> GIYQHFSIEDRPFLDKGMEWIKKVEDSYAPFLTPFINPHQEKLLKILAKTYGLACSSSGEFVSSEYVRVLLYPDYFQPEFSDFEISLQEIVYSNKFEYLTHAKILGTVINQLGIERKLFGDILVDEERAQIMINQQFLL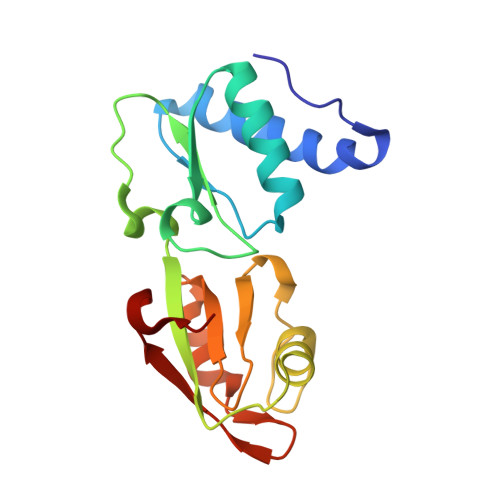LFQDGLKKIGRIPVSLEERPFTEKID> GPLGSMSLQEKLLTYYRNRAAIPAGEQARAKQAAVDICAELRSFLRAKLPDMPLRDMYLSGSLYDDLQVVTADHIQLIVPLVLEQNLWSCIPGEDTIMNVPGFFLVRRENPEYFPRGSSYWDRCVVGGYLSPKTVADTFEKVVAGSINWPAIGSLLDYVIRPAPPPEALTLEVQYERDKHLFIDFLPSVTLGDTVLVAKPHRLAQYDNLWRLSLRPAETARL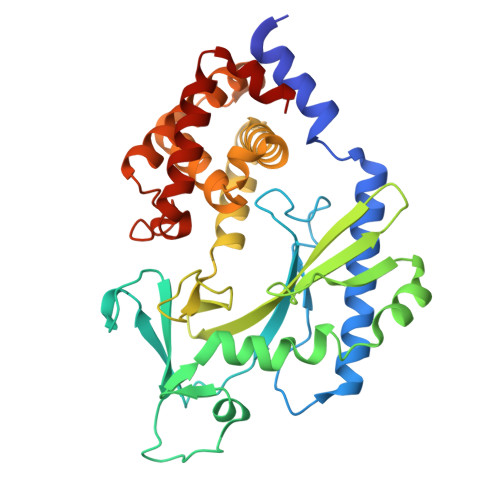RALDQADSGCRSLCLKILKAICKSTPALGHLTASQLTNVILHLAQEEADWSPDMLADRFLQALRGLISYLEAGVLPSALNPKVNLFAELTPEEIDELGYTLYCSLSEPEVLLQT>[6x]MDPMYLLVDVGNTHSVFSITEDGKTFRRWRLSTGVFQTEDELFSHLHPLLGDAMREIKGIGVASVVPTQNTVIERFSQKYF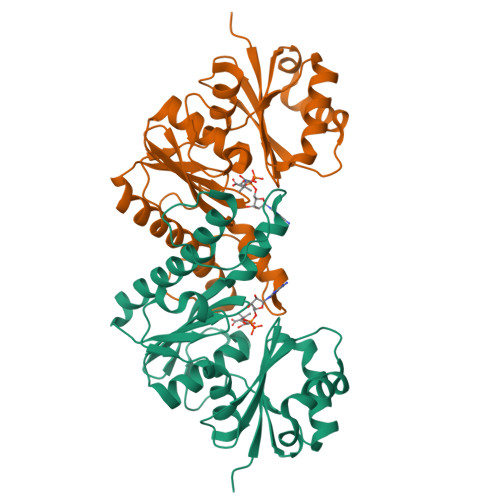HISPIWVKAKNGCVKWNVKNPSEVGADRVANVVAFVKEYGKNGIIIDMGTATTVDLVVNGSYEGGAILPGFFMMVHSLFRGTAKLPLVEVKPADFVVGKDTEENIRLGVVNGSVYALEGIIGRIKEVYGDLPVVLTGGQSKIVKDMIKHEIFDEDLTIKGVYHFCFGD>[2x]PVTLTLYNGQHAATGIAIAKAFQDKTGIQVKIRKGGDGQLASQITEEGARSPADVLYT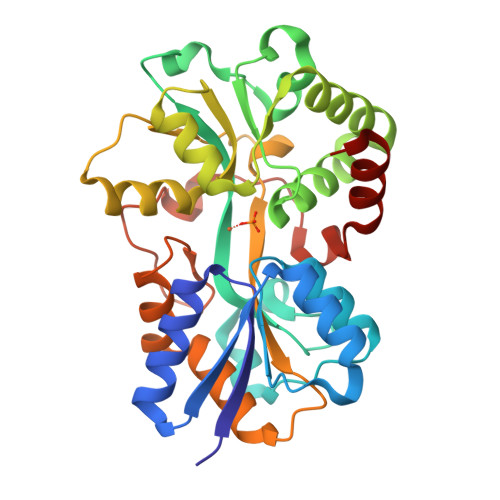EESPPLIRLASAGLLAKLEPETLALVEPEHAGGNGDWIGITARTRVLAYNPKKIDEKDLPKSLMDLSDPSWSGRFGFVPTSGAFLEQVAAVIKLKGQEEAEDWLTGLKAFGSIYTNNVTAMKAVENGEVDMALINNYYWYTLKKEKGELNSRLHYFGNQDPGALVTVSGAAVLKSSKHPREAQQFVAFMLSEEGQKAILSQSAEYPMRKGMQADPALKPFAELDPPKLTPADLGEASEALSLERDVGLN>[4x]PQFEKIE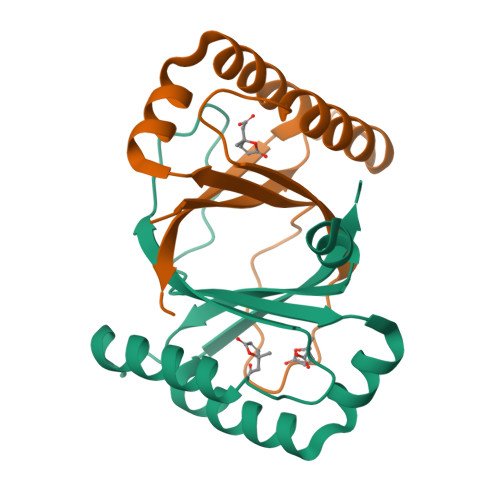GRMIRILYLLVKPESMSHEQFRKECVVHFQMSAGMPGLHKYEVRLVAGNPTDTAVPYLDVGRIDAIGECWFASEEQYQVYMESDIRKAWFEHGKYFIGQLKPFVTEELV>GPLGSENVEQIDAELVLSIEKLQEIQDDLEKINEKASDEVLEVEQKYNVIRKPVYDKRNEIIKTIPDFWLTAFLSHPALGELLTEEDQKIFKYLSSLDVEDAKDVKSGYSITFSFNPNPFFEDGKLTKTFTFLEEGTTKITATPIKWKEGKGLANGVNHEKNGNKRALPEESFFTWFSDAQHKEDVEDEMQDEQVADIIKEDLWPNPLTYFNNDA[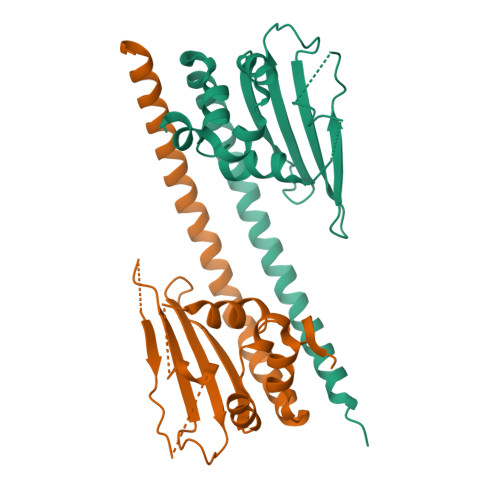2x]> GRPRAINKHEQEQISRLLEKGHPRQQLAIIFGIGVSTLYRYFPASSIKKR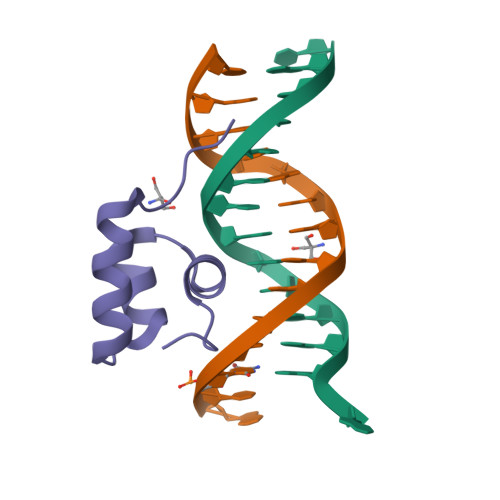MN>MASGSMHLRPIATPYPVKEWLQPKRYKAHLMGTTYVYDFPELFRQASSSQWKNFSADVKLTDDFFISNELIEDENGELTEVEREPGANAIGMVAFKITVKTPEYPRGRQFVVVANDITFKIGSFGPQEDEFFNKVTEYARKRGIPRIYLAANSGARIGMAEEIVPLFQVAWNDAANPDKGFQYLYLTSEGMETLKKFDKENSVLTERTVINGEERFVIKTIIGSEDGLGVECLRGSGLIAGATSRAYHDIFTITLVTCRSVGIGAYLVRLGQRAIQVEGQPIILTGASALNKVLGREVYTSNLQLGGTQIMYNNGVSHLTAVDDLAGVEKIVEWMSYVPAKRNMPVPILETKDTWDRPVDFTPTNDETYDVRWMIEGRETESGFEYGLFDKGSFFETLSGWAKGVVVGRARLGGIPLGVIGVETRTVENLIPADPANPNSAETLIQQAGQVWFPNSAFKTAQAINDFNNGEQLPMMILANWRGFSGGQRDMFNEVLKYGSFIVDALVDYKQPIIIYIPPTGELRGGSWVVVDPTINADQMEMYADVNARAGVLEPEGTVEIKFRREKLLDTMNRLDDKYRELRSQLSNKSLAPEVHQQISKQLADRERELLPIYGQISLQFADLHDRSSRMVAKGVISKELEWTEARRFFFWRLRRRLNEEYLIKRLSHQVGEASRLEKIARI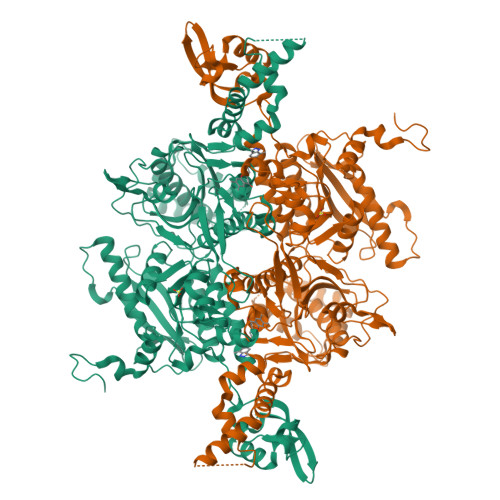RSWYPASVDHEDDRQVATWIEENYKTLDDKLKGLKLESFAQDLAKKIRSDHDNAIDGLSEVIKMLSTDDKEKLLKTLKLEHHHHHH[3x]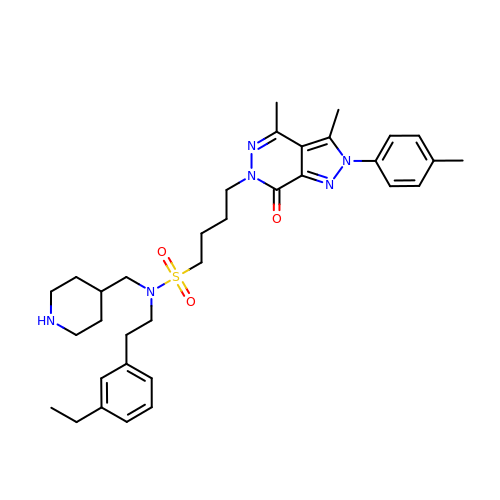4-[3,4-dimethyl-2-(4-methylphenyl)-7-oxidanylidene-pyrazolo[3,4-d]pyridazin-6-yl]-~{N}-[2-(3-ethylphenyl)ethyl]-~{N}-(piperidin-4-ylmethyl)butane-1-sulfonamide | C34 H46 N6 O3 S | QHFTYTSBWBJCGY-UHFFFAOYSA-N>PGMAGDSEQTLQNHQQPNGGEPFLIGVSGGTASGKSSVCAKIVQLLGQNEVDYRQKQVVILSQDSFYRVLTSEQKAKALKGQFNFDHPDAFDNELILKTLKEITEGKTVQIPVYDFVSHSRKEETVTVYPADVVLFEGILAFYSQEVRDLFQMKLFVDTDADTRLSRRVLRDISERGRDLEQIL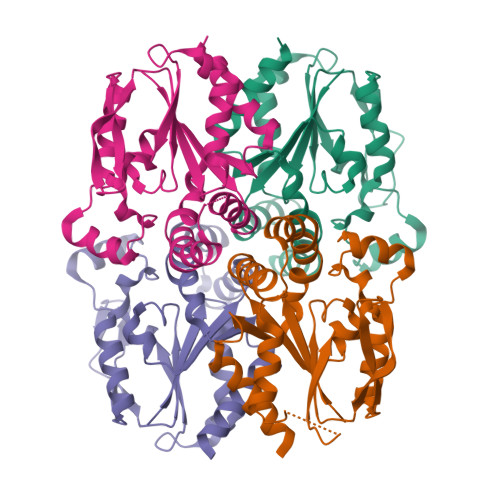SQYITFVKPAFEEFCLPTKKYADVIIPRGADNLVAINLIVQHIQDILNGGPSKRQTNGCLNGYTPSRK[4x]> SPLFAEPYKVTSK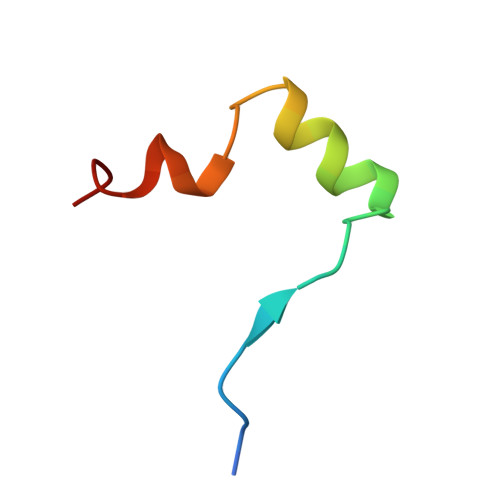EDKLSSRIQSMLGNYDEMKDFIG>[6x]MRGSHHHHHHGSMD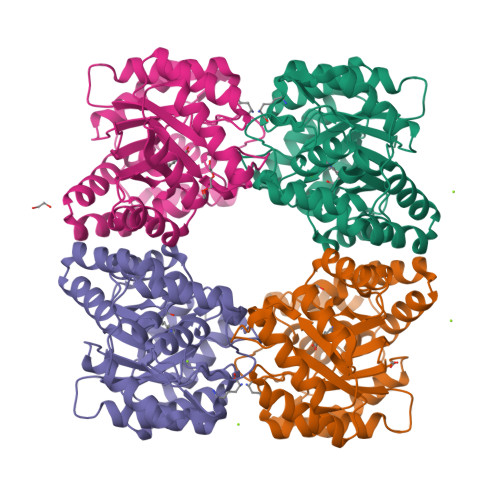KNIIIGAMTALITPFKNGKVDEQSYARLIKRQIENGIDAVVPVGTTGESATLTHEEHRTCIEIAVETCKGTKVKVLAGAGSNATHEAVGLAKFAKEHGADGILSVAPYYNKPTQQGLYEHYKAIAQSVDIPVLLYNVPGRTGCEISTDTIIKLFRDCENIYGVKEASGNIDKCVDLLAHEPRMMLISGEDAINYPILSNGGKGVISVTSNLLPDMISALTHFALDENYKEAKKINDELYNINKILFCESNPIPIKTAMYLAGLIESLEFRLPLCSPSKENFAKIEEVMKKYKIKGF> MAETEIHTFDDIPMPKLADPLLIYTPANEIFDIASCSAKDIGFAIAHAQIPPGGGPMPHIHYFINEWFWTPEGGIELFHSTKQYPNMDELPVVGGAGRGDLYSIQSEPKQLIYSPNHYMHGFVNPTDKTLPIVFVWMRNEVAPDFPYHDGGMREYFQAVGPRITDLNNLPELTNAQRAAFASEAPKYGINQSSYFMEYVNTISDKLPAQIAK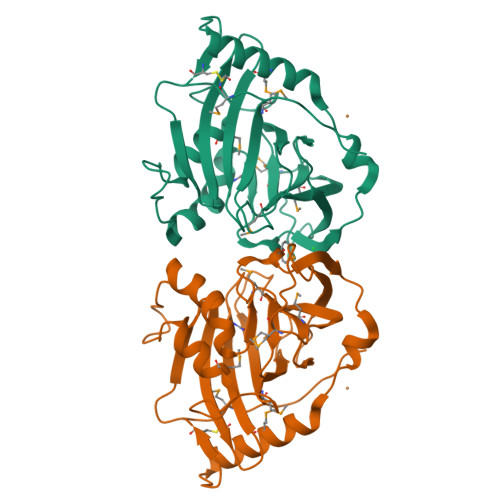LKNDKDLERMVEVIEAFNRGDKSVTCS> MAHHHHHHMLAIGITGSYASGKTFILDYLAEKGYKTFCADRCIKELYQDLSVQTQILKLLPELESFNIGKISNLIYNNDLAREKLQNFIYPLLIDKLILFKKENANSKFGFAEIPLLYEAKFDKYFDFVVTIYCSEEIRMQRAITRTSFDIEIYNKIKEIQLSQESKI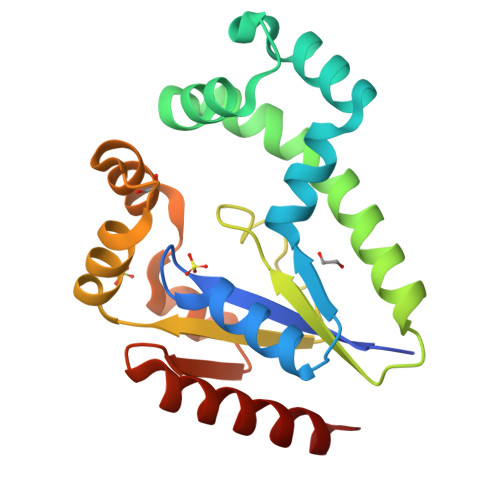AKADFAINSGVDMLDLEKQIEKLILVIARKL> K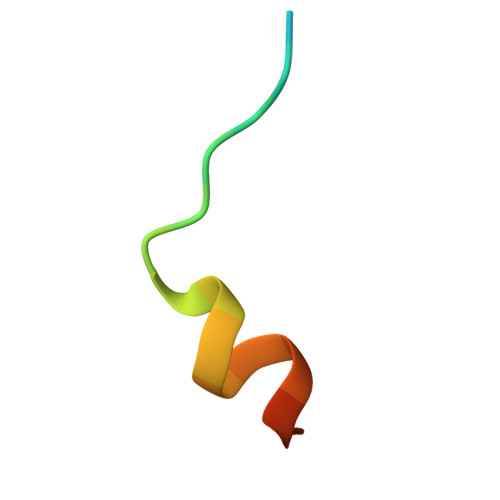ADLGPISLNWFEELSSEA>[6x]MTREDM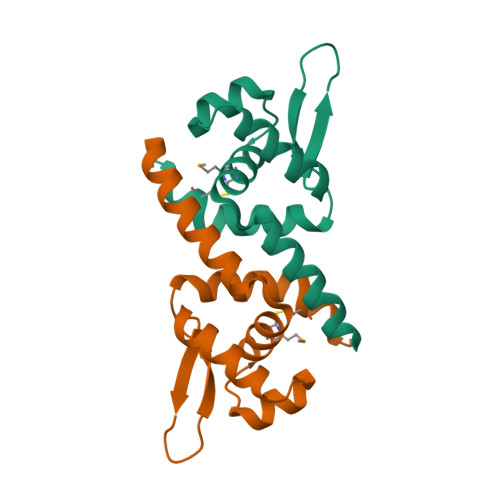EKRANEVANLLKTLSHPVRLMLVCTLVEGEFSVGELEQQIGIGQPTLSQQLGVLRESGIVETRRNIKQIFYRLTEAKAAQLVNALYTIFCAQEKQA> MSSERTFIAVKPDGVQRGLVGEIIARFERKGYKLVALKILQPTTEQAQGHYKDLCSKPFFPALVKYFSSGPIVCMVWEGKNVVK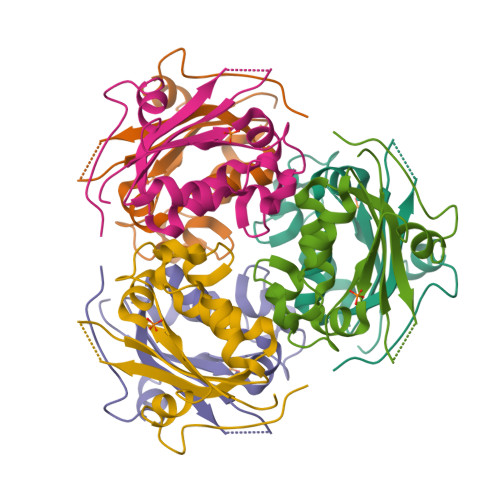SGRVLLGATNPADSQPGTIRGDFAVDVGRNVCHGSDSVESAEREIAFWFKADEIASWTSHSVSQIYE>MRGSHHHHHHGSELPQMVQQLNSPDQQELQSALRKLSQIASGGNEQIQAVIDAGALPALVQLLSSPNEQILQEALWALSNIASGGNEQIQAVIDAGALPALVQLLSSPNEQILQEALWALSNIASGGNEQIQAVIDAGALPALVQLLSSPNEQILQEALWALSNIASGGNEQKQAVKEAGAEPALEQLQSS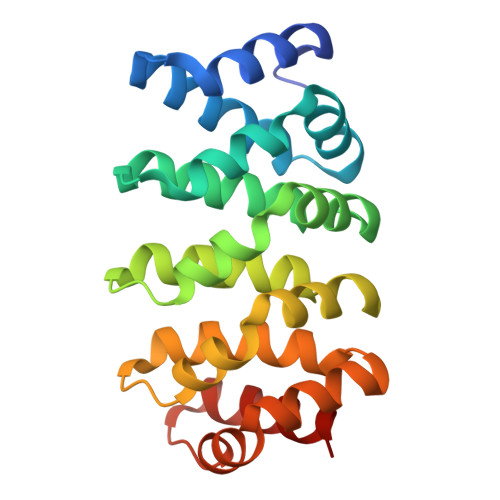PNEKIQKEAQEALEKIQSH[6x]> GSHMFC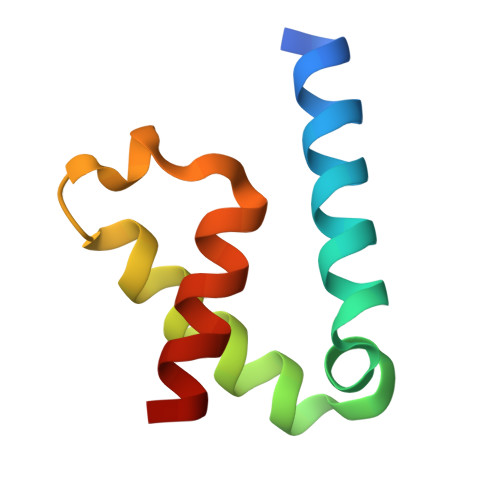EKYKQTKEQALTFFQEHPQYMRSKEDEEQLMTEFKKVLLEPGSKNLSIYQTLLAAHERLQAL>MGSDKIHHHHHHMKIDILDKGFVELVDVMGNDLSAVRAARVSFDMGLKDEERDRHLIEYLMKHGHETPFEHIVFTFHVKAPIFVARQWFRHRIASYNELSGRYSKLSYEFYIPSPERLEGYKTTIPPERVTEKISEIVDKAYRTYLELIESGVPREVARIVLPLNLYTRFFWTVNARSLMNFLNLRADSHAQWEIQQYALAIARIFKE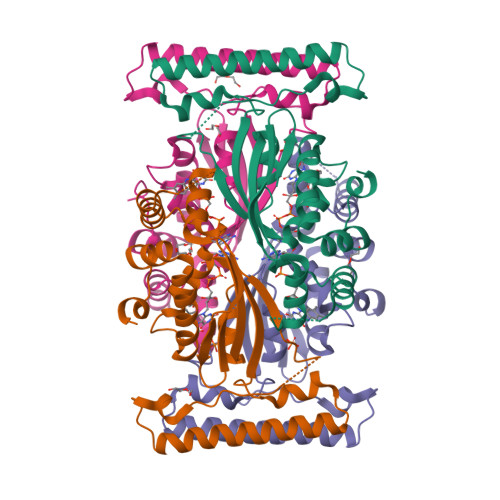KCPWTFEAFLKYAYKGDILKEVQV[4x]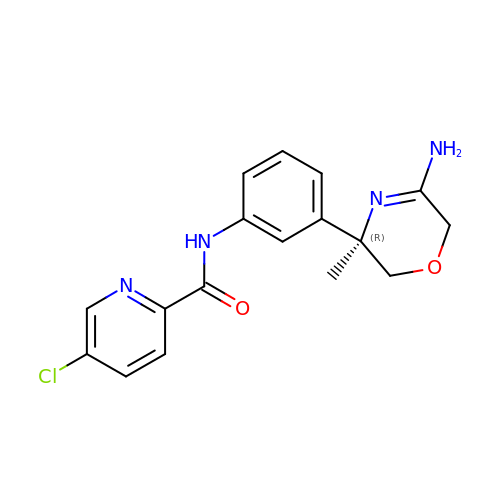N-{3-[(3R)-5-amino-3-methyl-3,6-dihydro-2H-1,4-oxazin-3-yl]phenyl}-5-chloropyridine-2-carboxamide | C17 H17 Cl N4 O2 | ZZUPAAPYPBQGKS-KRWDZBQOSA-N>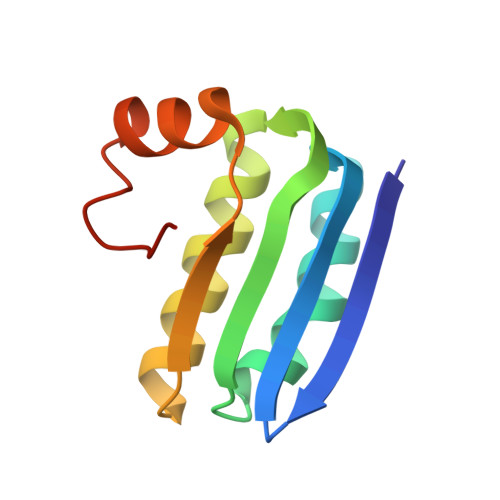 NINVDVKQNENDIQVNIAGEIDVYSAPVLREKLVPLAEQGADLRICLKDVSYMDSTGLGVFVGTFKMVKKQGGSLKLENLSERLIRLFDITGLKDIIDISAKS>[4x]MDLAKLGLKEVMPTKINLEGLVGDHAFSM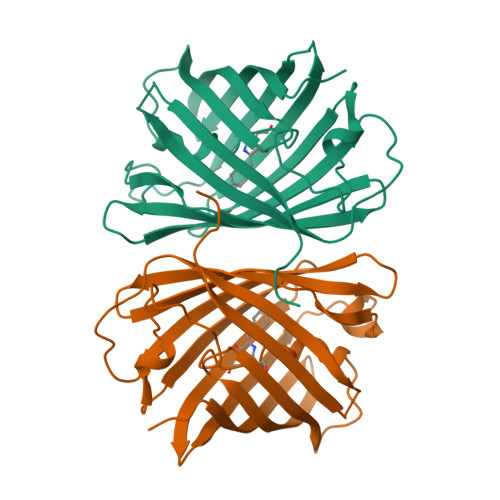EGVGEGNILEGTQEVKISVTKGAPLPFAFDIVSVAFTYGNRAYTGYPEEISDYFLQSFPEGFTYERNIRYQDGGTAIVKSDISLEDGKFIVNVDFKAKDLRRMGPVMQQDIVGMQPSYESMYTNVTSVIGECIIAFKLQTGKHFTYHMRTVYKSKKPVETMPLYHFIQHRLVKTNVDTASGYVVQHETAIAAHSTIKKIEGSLPVDHHHHHH>GMFASLVIPVSAQAN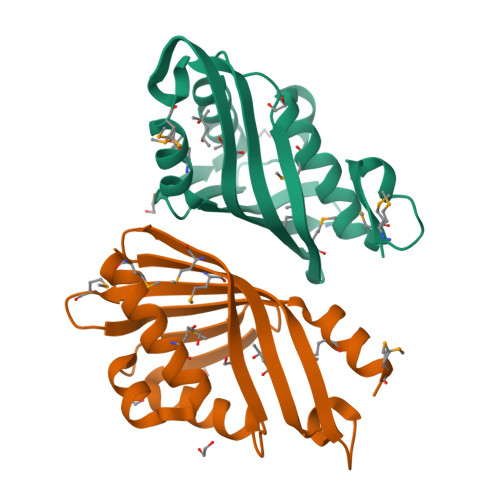SGEMPQEQQLAVKYMDALTEHDYKTLITFYNRDSIFFDKTANRKYTGGRFIIDFLERAHQGVLEYDFNIEHMYNAGSLVVMIGNYHFKGPGEQFGKPGKIIDVAIPAVTSLKLDMLNRRVTEHVDLIDYQTMSDQLAMQ[8x]> AWTQEKNHHQPAHLNSSSLQQVAEGTSISEMWQNDLRPLLIERYPGSPGSYSARQHIMQRIQRLQAEWVVEVDTFLSRTPYGYRSFSNIISTLNPEAKRHLVLACHYDSKYFPRWDSRVFVGATDSAVPCAMMLELARAL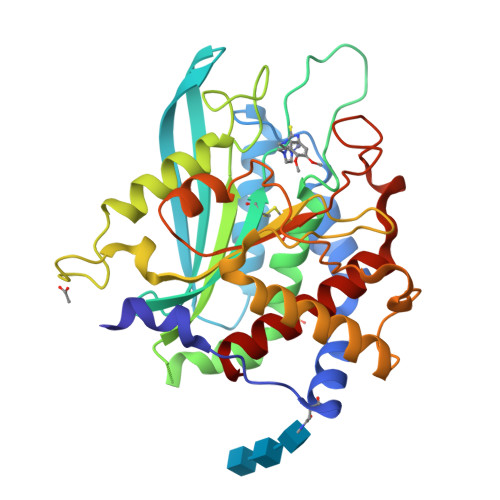DKKLHSLKDVSGSKPDLSLQLIFFDGEEAFHHWSPQDSLYGSRHLAQKMASSPHPPGSRGTNQLDGMDLLVLLDLIGAANPTFPNFFPKTTRWFNRLQAIEKELYELGLLKDHSLERKYFQNFGYGNIIQDDHIPFLRKGVPVLHLIASPFPEVWHTMDDNEENLHASTIDNLNKIIQVFVLEYLHL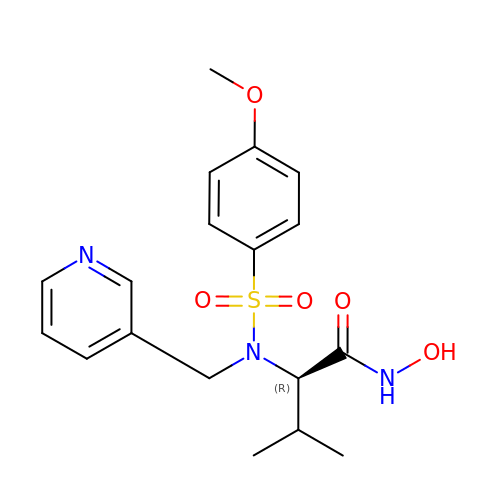N-HYDROXY-2(R)-[[(4-METHOXYPHENYL)SULFONYL](3-PICOLYL)AMINO]-3-METHYLBUTANAMIDE HYDROCHLORIDE | C18 H23 N3 O5 S | BSIZUMJRKYHEBR-QGZVFWFLSA-N> 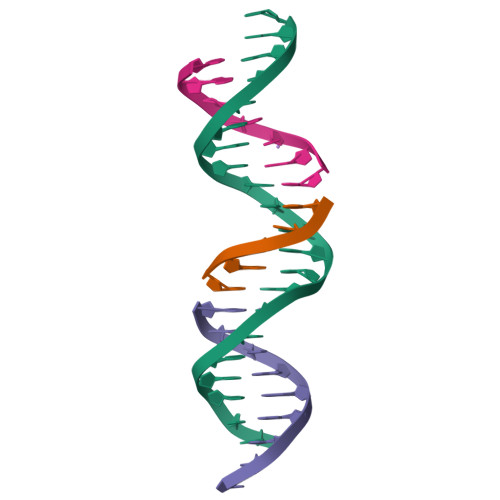GAGCAGACGTGACACCACTCA;> TGTCA;> TCTGAGTGG;> CGTCTGC>[2x]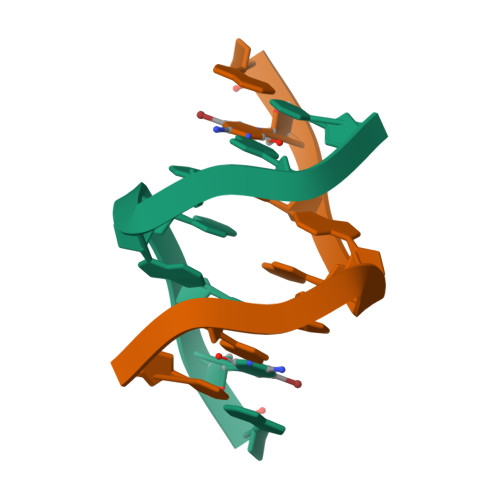GCGAACGC> FSEKPTTKSDVKIVEDILRGKKLKFKTDSGVFSYGKVDKGTKILVEN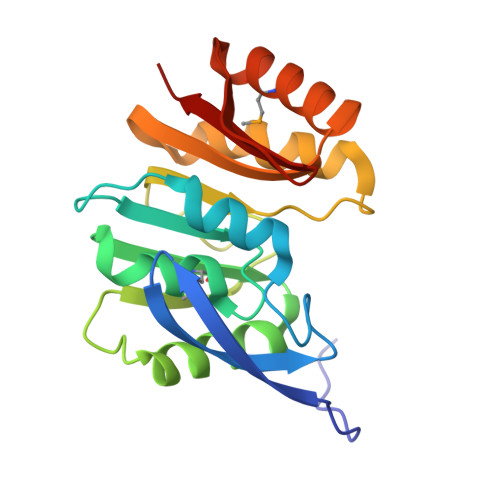VVVDKDDDILDLGCGYGVIGIALADEVKSTTMADINRRAIKLAKENIKLNNLDNYDIRVVHSDLYENVKDRKYNKIITNPPIRAGKEVLHRIIEEGKELLKDNGEIWVVIQTKQGAKSLAKYMKDVFGNVETVTIKGGYRVLKSKKL> GSHMKNSVSVDLPGSMKVLVSKSSNADGKYDLIATVDALELSGTSDKNNGSGVLEGVKADASKVKL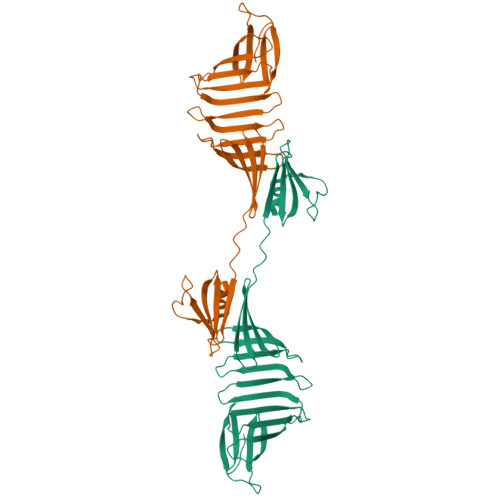TISDDLGQTTLEVFKSDGSTLVSKKVTSKDKSSTEEKFNEKGEVSEKIITRADGTRLEYTGIKSDGSGKAKEVLKGYVLEGTLTAEKTTLVVKEGTVTLSKNISKSGAVSVELNDTPPPPPPKKTAAWNSGTSTLTITVNSKKTKDLVFTSSNTITVQQYDSNGTSLEGSAVEITKLDEIKNALK> GEFAQECQNLEVERQRRLERIKQKQSQLQELILQQIAFKNLVQRNRHAEQQASRPPPPNSVIHLPFIIVNTSKKTVIDCSISNDKFEYLFNFDNTFEIHDDIEVLKRMGMAC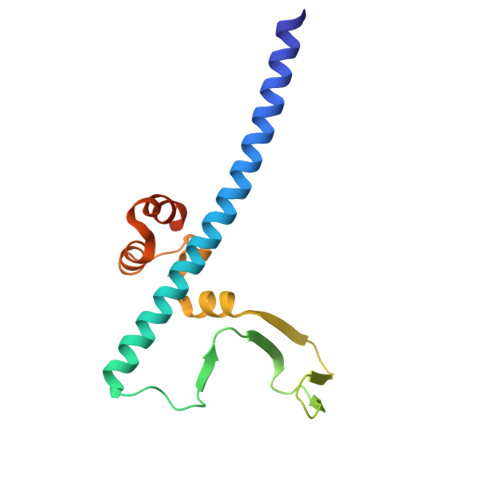GLESGSCSAEDLKMARSLVPKALEPYVTEMAQGTVGGVFITTA> UCCCAGUCCACCG;> CGGUGAIAAGGG;> 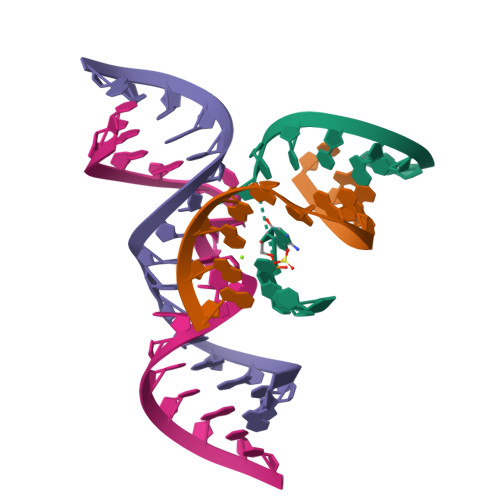GGCAGAGAAACACACGA;> UCGUGGUACAUUACCUGCC>[4x]MKITVIGAGNVGATTAFRLAEKQLARELV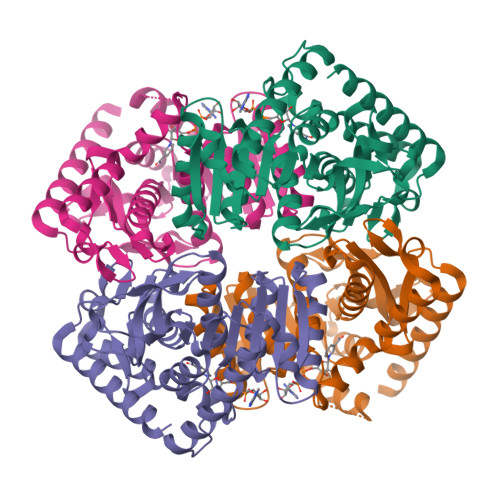LLDVVEGIPQGKALDMYESGPVGLFDTKVTGSNDYADTANSDIVIITAGLPRKPGMTREDLLMKNAGIVKEVTDNIMKHSKNPIIIVVSNPLDIMTHVAWVRSGLPKERVIGMAGVLDAARFRSFIAMELGVSMQDINACVLGGHGDAMVPVVKYTTVAGIPISDLLPAETIDKLVERTRNGGAEIVEHLKQGSAFYAPASSVVEMVESIVLDRKRVLPCAVGLEGQYGIDKTFVGVPVKLGRNGVEQIYEINLDQADLDLLQKSAKIVDENCKMLESTIG~{N}-cyclohexyl-2-phenoxy-ethanamide | 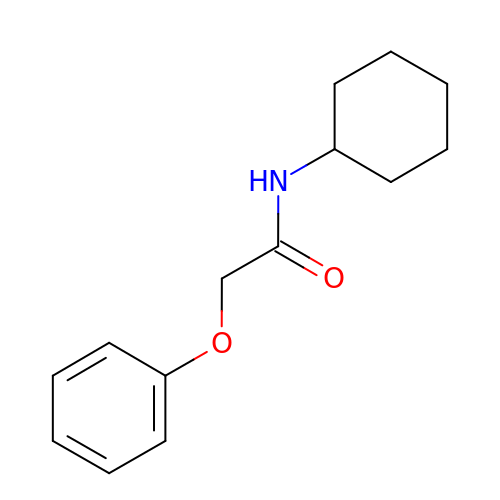C14 H19 N O2 | CQWWLWGATIFQLU-UHFFFAOYSA-N>[2x]QTIKDFLAVAMKKWTAPFEPFQLIDNIYYVGTDGIAVYVIKTSQGLILMDTAMPQSTGMIKDNIAKLGFKVADIKLILNTHAHLDHTGGFAEIKKETGAQLVAGERDKPLLEGGYYPGDEKNEDLAFPAVKVDRAVKEGDRVTLGDTTLTAHATPGHSPGCTSWEMTVKDGKEDREVLFFCSGTVALNRLVGQPTYAGIVDDYRATFAKAKAMKIDVLLGPHPEVYGMQAKRAEMK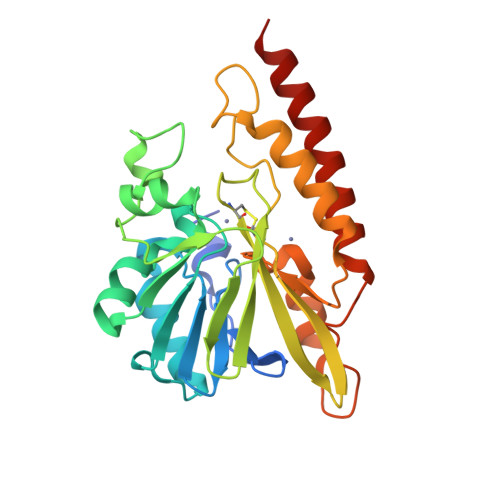DGAPNPFIKPGELVTYATSLSEDFDKQLAKQTAALEKK>[3x]MSLPRPAGHEADGAAAADAKPVWDLPVHGEPWERPDGELVRSLNRVSSATACAKLHE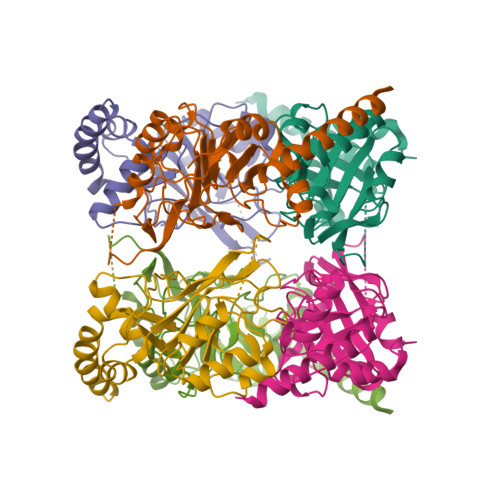LGIRRSYLSGPTALDLGNKVTGPARTLQFMPQREDVASGLAQEYVERSTALWAVLEEVQPGDVLVVQAYGSAFTGCLGDMLVRYFKRKGGAGIVVDGRIRDAPRVRELGVPIWCTGTTPHYASQSELFPWAYDVPVAAGGVLTLPGDLVVADDDGAVVVPVSKAQEIVDSAFDHEQWEEFSRMRIDQGARLSDYYPLSPDSREEYEQWRASKR>[2x]MTIKPAVRISDGNLIIKNRTILTGVPDNVITTSASEAGPVEGVFVGAVFNKEESKHIVPIGTLRNSRFMSCFRFKLWWMAQRMGEMGRDIPYETQFLLVESNDGSHLESDGANGVECNQKVYTVFLPLIE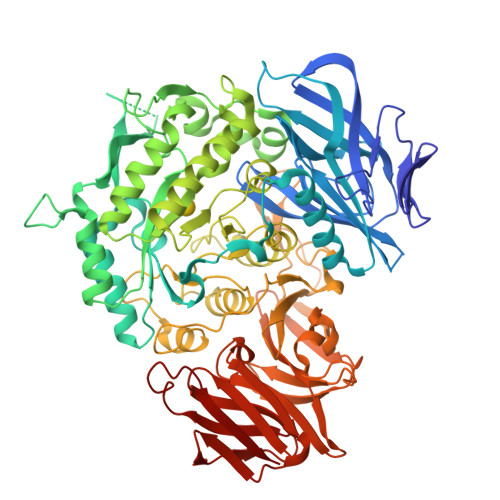GSFRSCLQGNVNDEVELCLESGDVDTKRSSFTHSLYIHAGTDPFQTITDAIRTVKLHLNSFRQRHEKKLPGIVDYFGWCTWDAFYQEVTQEGVEAGLKSLAAGGTPPKFVIIDDGWQSVERDATVEAGDEKKESPIFRLTGIKENEKFKKKDDPNVGIKNIVKIAKEKHGLRYVYVWHAITGYWGGVRPGEEYGSVMKYPNMSKGVVENDPTWKTDVMTLQGLGLVSPKKVYKFYNELHSYLADAGVDGVKVDVQCVLETLGGGLGGRVELTRQFHQALDSSVAKNFPDNGCIACMSHNTDALYCSKQAAVIRASDDFYPRDPVSHTIHIASVAYNSVFLGEFMQPDWDMFHSVHPAAEYHASARAISGGPLYVSDSPGKHNFELLRKLVLPDGSILRARLPGRPTRDCLFADPARDGVSLLKIWNMNKYTGVLGVYNCQGAAWSSTERKNIFHQTKTDSLTGSIRGRDVHSISEASTDPTTWNGDCAVYSQSRGELIVMPYNVSLPVSLKIREHEIFTVSPISHLVDGVSFAPIGLVNMYNSGGAIEGLRYEAEKMKVVMEVKGCGKFGSYSSVKPKRCVVESNEIAFEYDSSSGLVTFELDKMPIENKRFHLIQVEL(1R)-3-amino-1-[3-(cyclohexylmethoxy)phenyl]propan-1-ol 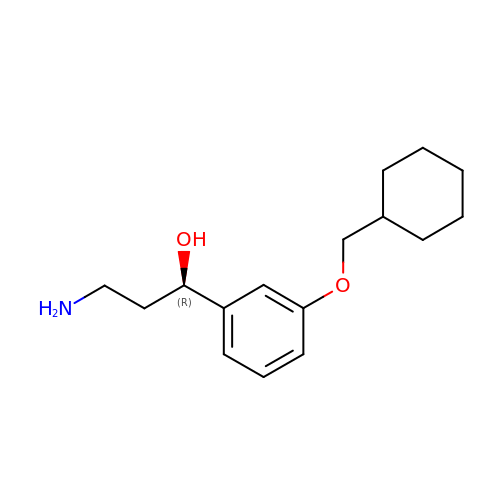| C16 H25 N O2 | WJIGGYYSZBWCGC-MRXNPFEDSA-N>HHHSQDPMYLKEIFVDNFRNLKKQKLEFCEGVNLIYGLNAQGKSNLLEAIRLLSMGRSFRGSKMSELVKFDEEYFYVRGLVRSADFYEKKIEFGYKVNGNKVIKVNGNKLKSTGEILGHFLTVIFSPEDIEIIKEGPSRRRKYLDACISVIDKNYFFDLLQYNKTLSNRNSLLKKIKEEGKGEDLLEIFDEKLAEYGARIIKVRNNYLEKLKNSMSKFLMEISNEKLEIIYLNSAGVKEVHEENLIREKLKNRL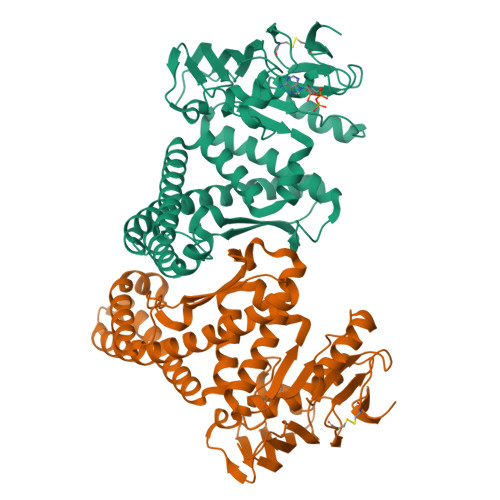TKSLTLDLKYLSTQVGPHREDFKILINGYDSRVYSSQGQKRTAALCLKLSELEILEEETGEKPVLLLDDVMSELDDNRKKYILKKLEGFQSFITHTSKSDVEGDCCFKIYDGIVDKLA[2x]> GSAYSEKVIDHYENPRNVGSFDNNDENVGSGMVGAPACGDVMKLQIKVNDEGIIEDARFKTYGCGSAIASSSLVTEWVKGKSLDEAQAIKNTDIAEELELPPVKIHCSILAEDAIKAAIADYKSKREAK;> MGSSHHHHHHGSMYGVYRAMKLPIYLDYSATTPVDPRVAEKMMQFMTMDGTFGNPASRSHRFGWQAEEAVDIARNQIADLVGADPREIVFTSGATESDNLAIKGAANFYQKKGKHIITSKTEHKAVLDTCRQLEREGFEVTYLAPQRNGIIDLKELEAAMRDDTILVSIMHVNNEIGVVQDIAAIGEMCRARGIIYHV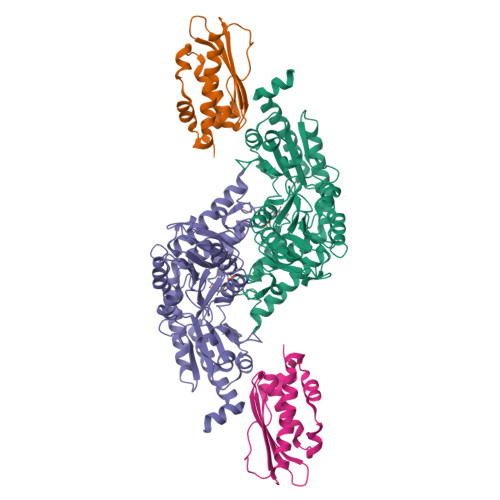DATQSVGKLPIDLSQLKVDLMSFSGHKIYGPKGIGALYVRRKPRVRIEAQMHGGGHERGMRSGTLPVHQIVGMGEAYRIAKEEMATEMERLRGLRNRLWNGIKDIEEVYLNGDLEHGAPNILNVSFNYVEGESLIMALKDLAVSSGSACTSASLEPSYVLRALGLNDELAHSSIRFSLGRFTTEEEIDYTIELVRKSIGRLRDLSPLWEMYKQGVDLNSIEWAHH> GSMSVLSIVTVPDKRLSLCSEEVEKVDQSIRKLVDDMFETMHANQGLGLAAVQVGVHKRI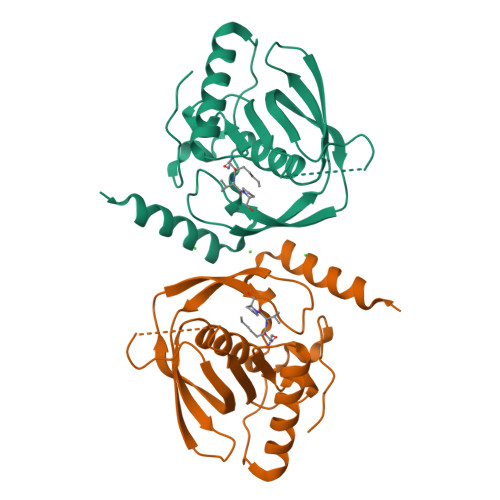LVMNVPEEFEDSEDIENVEDKIEGYELYGGPYCIINPKIVDISQEKVKLKEGCLSVPGYFDYIVRPQRIAVQYLDYNGNECIIKAQGWLARCLQHEIDHLNGTVFLKYLSKFKRDFAIEKVKKKERTDLI>MDMTQQEIFDKQRRLQELSEKVRTCHQEASALRKALQEKEAEM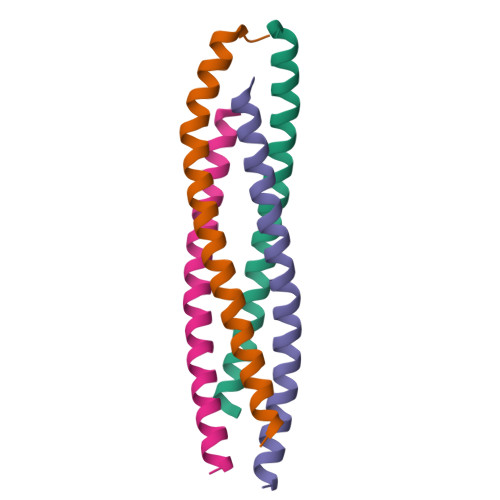LQVLEDIQTI[4x]>[2x]MQKNLDSLLENLRAEIDA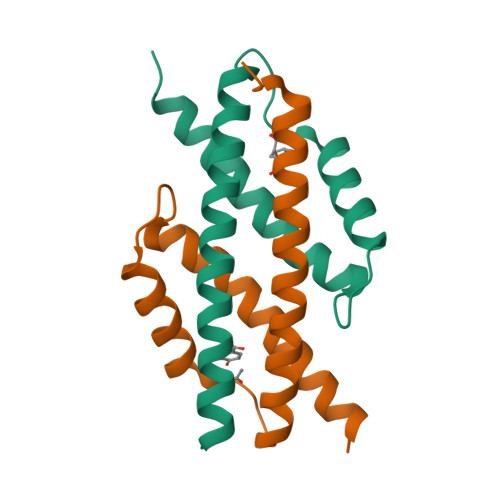LDNELSDLLDKRLEIALKIALIKQESPIYCPKREQEILKRLSQRDFKHLNGEILTGFYTEVFKISRKFQENALKELKK(2R,3R,4S,5R,6R)-3,5-dihydroxy-4-[(E)-({3-hydroxy-2-methyl-5-[(phosphonooxy)methyl]pyridin-4-yl}methylidene)amino]-6-methyltetrahydro-2H-pyran-2-yl 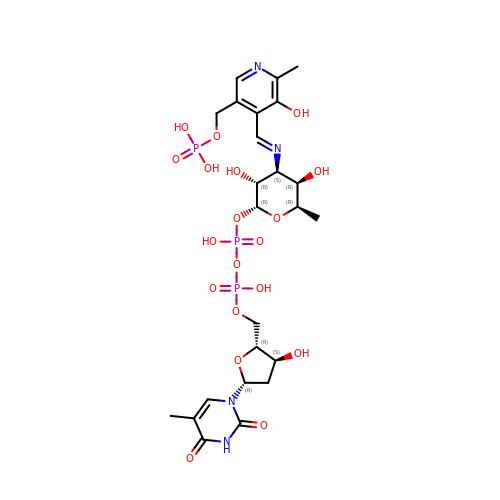[(2R,3S,5R)-3-hydroxy-5-(5-methyl-2,4-dioxo-3,4-dihydropyrimidin-1(2H)-yl)tetrahydrofuran-2-yl]methyl dihydrogen diphosphate (non-preferred name) | C24 H35 N4 O19 P3 | UJDWKFAFGYHSFM-QBLVGKJYSA-N N-[(1S)-1-BENZYL-2,2-DIHYDROXY-3-(TETRAHYDRO-2H-PYRAN-4-YLAMINO)PROPYL]-6-ETHYL-1-METHYL-1,3,4,6-TETRAHYDRO[1,2]THIAZEPINO[5,4,3-CD]INDOLE-8-CARBOXAMIDE 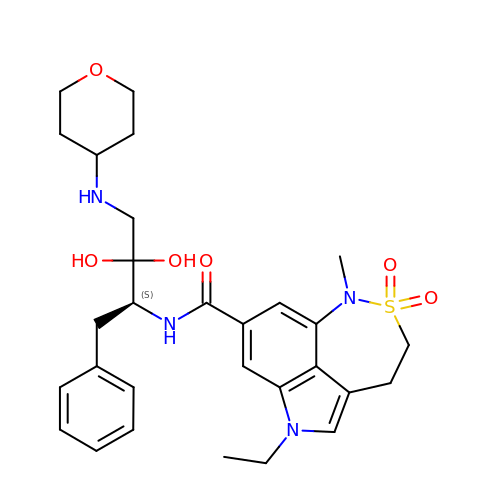2,2-DIOXIDE | C29 H38 N4 O6 S | LMEDJLLRHRUTJN-SANMLTNESA-N>GXCCCGGGAC[2x]

Oligodeoxynucleotides incorporating internucleotide phosphoroselenolate linkages have been prepared under solid-phase synthesis conditions using dimer phosphoramidites. Replacement of a bridging oxygen (3′ or 5′) within an internucleotide phosphate diester by selenium gives rise to phosphoroselenolate analogues. These are achiral and potentially more stable than the corresponding phosphoroselenoates but have been documented in only a very limited number of communications. The phosphoroselenolate linkage was found to impart resistance to nuclease activity.

To confirm that the structure of the nucleic acid is not significantly perturbed by the introduction of a phosphoroselenolate modification, crystallisation trials of oligodeoxynucleotide sequences containing the group were performed. This resulted in the crystal structure of d(GSeTCCCGGGAC) – ODN 4 – being obtained, which allows for visualisation of the modification at 1.45 Å resolution. The structure shows that the overall conformation of the duplex is that of A-DNA. The average twist of the helix is 31.8° which compares favourably to a standard value of 32.7°. However, at the modification site the T*–A base pair has a twist of ca. 41°, which can be attributed to the increased bond lengths from P–Se (2.25 Å) and Se–C5′ (1.94 Å) compared to the oxygen-containing equivalent (P–O5′ 1.60 Å, O5′–C5′ 1.42 Å). Apart from this slight increase in bond lengths, and subsequent increase in helical twist angle, the base pair containing the phosphoroselenolate modification is otherwise consistent with a standard A-DNA base pair, with parameters such as roll, tilt, rise and slide all within the normal range for this conformation (analysis performed using W3DNA). Whilst it could be expected that the increased twist or bond lengths could affect the sugar pucker of the nucleotide, this is not the case, with the nucleotide possessing a C3′-endo sugar pucker, consistent with that of A-DNA. The nucleotide 3′ to the modified base also possesses a C3′-endo pucker. The base 5′ to the modification site possesses a non-standard pucker, C2′-exo, which is attributed to the proximity of a neighbouring strand, forming a crystal contact within the lattice. This structure therefore confirms that the introduction of the modification does not significantly perturb the solid-state conformation of the duplex.Here we report the discovery of a multichaperone condensate in the ER lumen, which is formed around the chaperone PDIA6 during protein folding homeostasis. PDIs contain one or more catalytically active thioredoxin-like domains, which can reduce, oxidize or isomerize disulfide bonds in client proteins via a characteristic CXXC motif. PDIA6 consists of two catalytically active thioredoxin-like domains, domains a0 and a, which are followed by the inactive domain b of unknown function. The PDIA6 condensates recruit further chaperones—Hsp70 BiP, J-domain protein ERdj3, disulfide isomerase PDIA1 and Hsp90 Grp94—which constitute some of the essential components of the early folding machinery.

The dimeric domain a0 is connected to domain a by a long positively charged linker, and domains a and b are connected by a short five-residue linker that presumably restricts the relative domain motions as it contains three conserved proline residues. Domains a and b unfold cooperatively, suggesting that they are stabilized by interdomain interactions. Titration of the paramagnetic analogue Gd3+, however, quenched NMR signals specifically in three structural regions, thus revealing three cation binding sites (I, II and III). Binding sites I and II are located at the domain a–b interface and in domain b, respectively. Taken together, the Ca2+-dependent phase separation of PDIA6 is controlled by a molecular switch in domain b, which is activated following Ca2+ binding. The data thus suggest a functional model for PDIA6 condensate formation, where the positively charged a0–a linker dynamically interacts with the negatively charged surface in domain b at homeostatic Ca2+ concentrations. The multivalency required for PDIA6 condensate formation thus results from (1) the high-affinity dimerization of domain a0 and (2) the transient Ca2+-dependent electrostatic interaction between the a0–a linker and domain b. PDIA6 interacts via its domain b with the nucleotide binding domain (NBD) of BiP. Importantly, the BiP binding site on domain b does not overlap with the interface required for condensate formation such that condensate formation and BiP recruitment by PDIA6 is simultaneously possible, as observed in cells.

> MGSSHHHHHHSSGENLYFQSPPPELLEIINEDIAKRTCEEHQLCVVAVLPHILDTGAAGRNSYLEVLLKLADKYKKKMWGWLWTEAGAQSELETALGIGGFGYPAMAAINARKMKFALLKGSFSEQGINEFLRELSFGRGSTAPVGGGAFPTIVEREPWDGRDGELPVEDDIDL4-cyclopentyl-N-[(1S,3R)-5-oxidanyl-2-adamantyl]-2-[[(3S)-oxolan-3-yl]amino]pyrimidine-5-carboxamide | C24 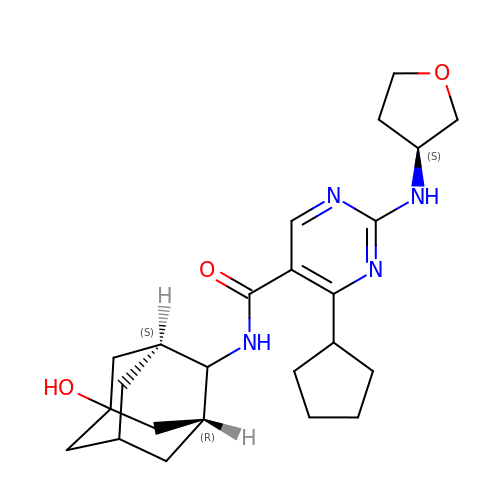H34 N4 O3 | VMTZDIHMLVWUQZ-GXLRSYGRSA-N10-oxohexadecanoic acid | C16 H30 O3 | 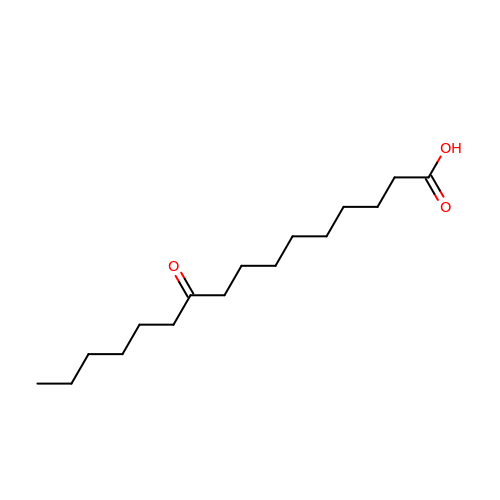VBFPQNKLKQDSCH-UHFFFAOYSA-N> GPPGPPG;> PGPPGPP;> PPGP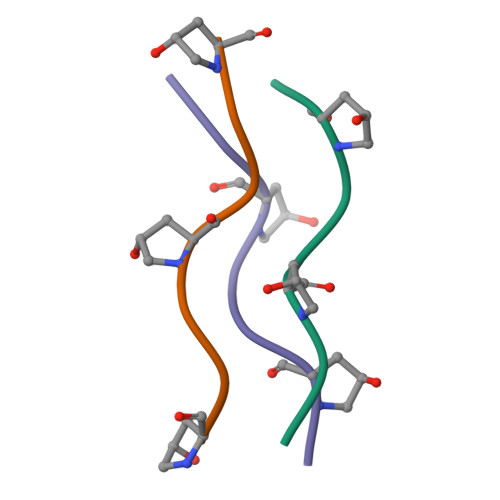PGP> GGAGUAGGCGUUGCGCAUUUUGUUGCUCAAAAGGCGACGAAACGCAAGGCAAUGCACGUCUGCGAUACACGAAAACAAUGCUAUUUGUUGAAAAUAUUGGAAUAAAGCAAAAGUCAUUGCCCGUCGCAAACGAAAGUGUGCUUCGGUAGCUAGGCUACCUGCUAGAGUCUCGCAAGGAUAAUAGCAAAGUCAAAGAGUAAAGCAGCUUAG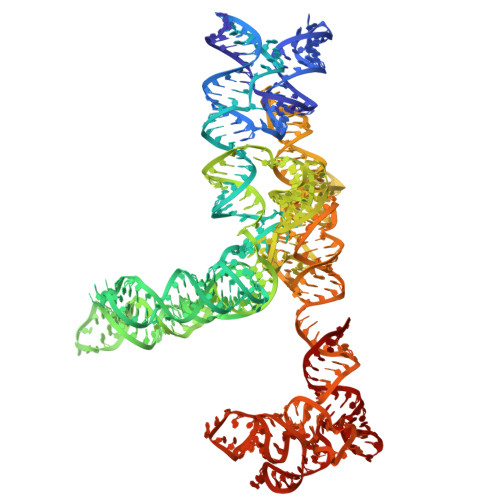ACCUUUAGCGGGGUUUUCGUUAAUUGAAAAAUGGCUUAGUAGUUUGCGGCGUAACGAGUGGUUAGCGAUACUAACCGCGCAUGGUUGUUACUUGAAGGGAUUUGAGUGGAUAAAAAACUAAAACAUAAGGUUUUGAAAGACAACUGACUAAACGUGUAAUCUCAGCGUAUUUGCAUUUGGAAAGUUACUCAAGUGGUUUAAGAGGACAGGUUGCUACCUUGUUAGGCGUGUAAAAGCGUGCGUGGGUUCGAAUCCUACACUUUCUA>MEEPEEPADSGQSLVPVYIYSPEYVSMCDSLAKIPKRASMVHSLIEAYALHKQMRIVKPKVASMEDMATFHTDAYLQHLQKVSQEGDDDHPDSIEYGLGYDCPATEGIFDYAAAIGGATITAAQCLIDGMCKVAINWSGGWHHAKKDEASGFCYLNDAVLGILRLRRKFERILYVDLDLHHGDGVEDAFSFTSKVMTVSLHKFSPGFFPGTGDVSDVGLGKGRYYSVNVPIQDGIQDEKYYQICESVLKEVYQAFNPKAVVLQLGADTIAGDPMCSFNMTPVGIGKCLKYILQWQLATLILGGGGFNLANTARCWTYLTGVILGKTLS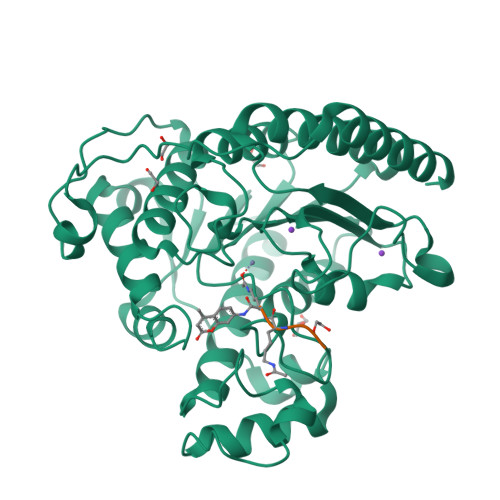SEIPDHEFFTAYGPDYVLEITPSCRPDRNEPHRIQQILNYIKGNLKHVVIEGRGSHHHHHH[2x]> GSHMGRRGWDNKASGTIRFGEGPSARSVWQASKDEATLEAIRVAGEDGAVPRPTRVAVAPEAEAMGDDDNEGQERDPIWVSWSNAMHSLRVGDIDAAYAEVLCAGDQHLVIKLMDKTGPSLDQMSNEIANEALNFISQFLLDHSLYDICLSWSQ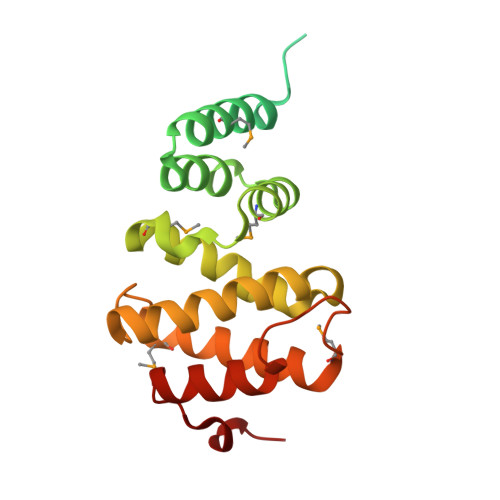QLLELVLQDGADTFGVPMELKTEILYNLQDACSTMDPPEDWEGPAPEQLVVQLASVWEIDLQQFDK> MQVIRKHLAQKGLFNPFLFNRFSTQQDITSVPGDKPPAIEDSIHGKYAGVLFSSASSNKSLNKVAEDMKYFNQLYKESEVFKSFLNNVSLKRNQQRDIISALGKTNFNP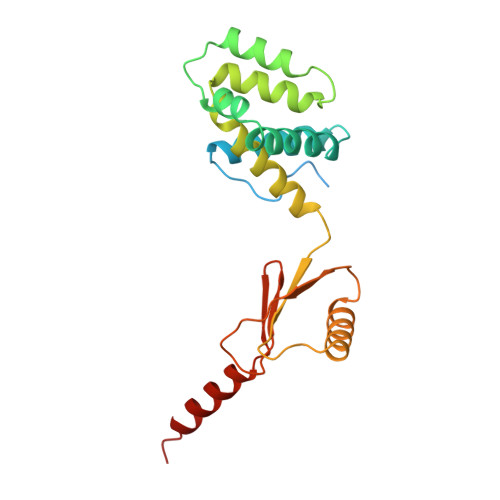ATNNLLETLIENKRLDSLPKIAEKYMDYYRILNKQESITIISAQELTAAEKQKVEQGLKKGNANVQFTVVYQVDPAILGGLQMYSGNNFLDCSLLSRVNKLKTEIAKISF1-[(1~{R},2~{R},4~{S},5~{S})-2,4-bis(4-carbamimidamidophenoxy)-5-[(4-carbamimidamidophenyl)amino]cyclohexyl]guanidine 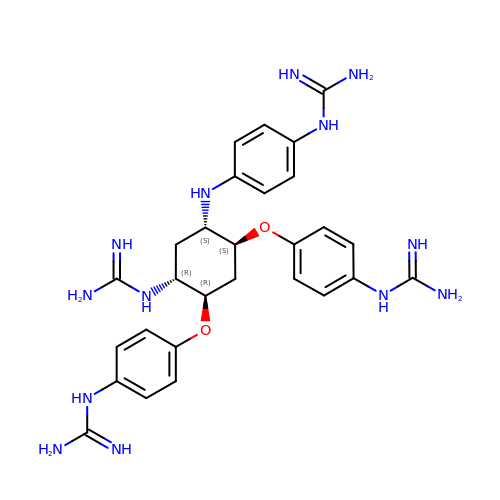| C28 H37 N13 O2 | PKMXMBXOZUEHDV-UARRHKHWSA-N>[4x]DTMKVINDPIHGHIELHPLLVRIIDTPQFQRLRYIKQLGGGYY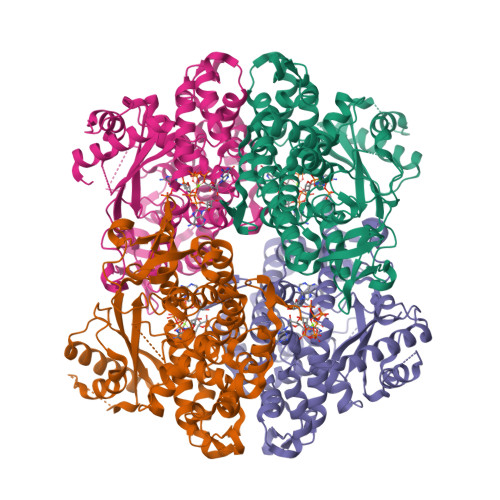VFPGASHNRFEHSLGVGYLAGCLVHALGEKQPELQISERDVLCVQIAGLCRNLGHGPFSHMFDGRFIPLARPEVKWTHEQGSVMMFEHLINSNGIKPVMEQYGLIPEEDICFIKEQIVGPLESPVEDSLWPYKGRPENKSFLYEIVSNKRNGIDVDKWDYFARDCHHLGIQNNFDYKRFIKFARVCEVDNELRICARDKEVGNLYDMFHTRNSLHRRAYQHKVGNIIDTMITDAFLKADDYIEITGAGGKKYRISTAIDDMEAYTKLTDNIFLEILYSTDPKLKDAREILKQIEYRNLFKYVGETQPTGQIKIKREDYESLPKEVASAKPKVLLDVKLKAEDFIVDVINMDYGMQEKNPIDHVSFYCKTAPNRAIRITKNQVSQLLPEKFAEQLIRVYCKKVDRKSLYAARQYFVQWCADRNFTKPQDGDVIAPLIEPQKKEWNDSTSVQNPTRLREASKSRVQLFKDDPM> TQTQLAIDNVLASAESTIQLNELPKVVLDFITGEQTSVARSGGIFTKEDLINLKLYVRKGLSLPTRQDEVEAYLGYKKIDVAGLEPKDIKLLFDEIHNHALNWNDVEQAVLQQSLDLDIAAKNIISTGNEIINLINQMPITLRV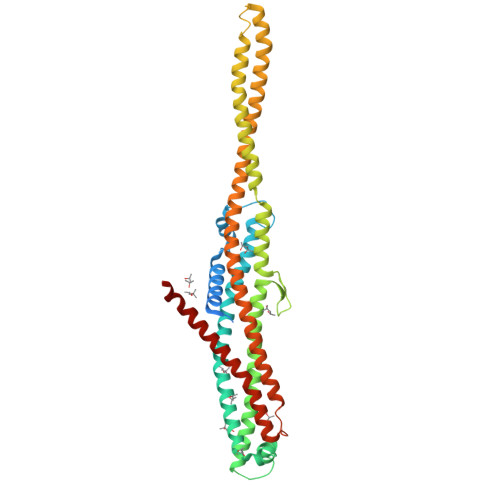KTLLGDITDKQLENITYESADHEVASALKDILDDMKGDINRHQTTTENVRKKVSDYRITLTGGELSSGDKVNGLEPQVKTKYDLMEKSNMRKSIKELDEKIKEKRQRIEQLKKDYDKFVGLSFTGAIGGIIAMAITGGIFGAKAENARKEKNALISEVAELESKVSSQRALQTALEALSLSFSDIGIRMVDAESALNHLDFMWLSVLNQITESQIQFAMINNALRLTSFVNKFQQVITPWQSVGDSARQLVDIFDEAIKEYKKVYG>[4x]MHHHHHHMNQLTILEAGLDEI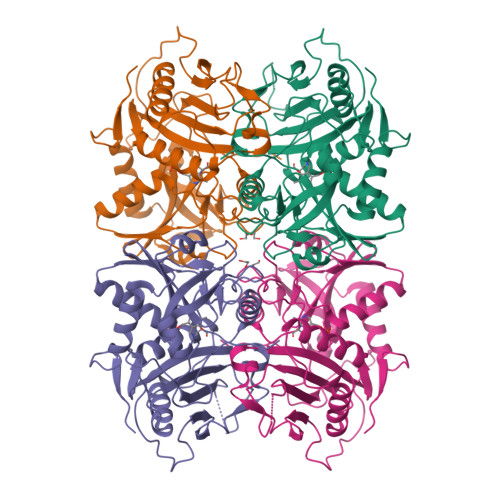ICETVPGEAIQYSRYSLDRTSPLAGGCAWIEGAFVPAAAARISIFDAGFGHSDVTYTVAHVWHGNFFRLEDHVERFLAGAEKMRIPMPATKAEIMDLMRGCVSKSGLREAYVNVCVTRGYGRKPGEKTLEALESQLYVYAIPYLWVFSPIRQIEGIDAVIAQSVRRSPANVMDPWIKNYQWGDLVRATFEAQERGARTAFLLDSDGFVTEGPGFNVLMVKDGTVFTAARNVLPGITRRTALEIARDFGLQTVIGDVTPEMLRGADEIFAATTAGGVTPVVALDGAPVGAGVPGDWTRKIRTRYWQMMDEPSDLIEPVSYI>MKKQFATMLAATAVLGVTTAFAANPFSDVTPDSWAYQAVSQLAQAGIVNGYPDGTFKGQNNITRYEMAQMVAKAMANQDRANAEQQAMINRLADEFSNELNNLGVRVSRLEDRVGNVKVTGDARIRYQGSEDKGVYKANSKSLTDGRARVQFNANVNDKTQAVVRVKGNYEFGDSTKGSQATIDRAYVDHKFGSNVSAKAGRFQQTIGGGLMYDDTFDGAQLNVGNDKVQVQGAYGYMIDGAADGNSKSDNPSVSYVGLKGKVGKESSVGGFYSRLSSGNLNHNGVTVNSDKQDVYGFNADFRKNKLWAGGEWLKASNVDNSQAWTAGLGYGNYDIAKKGTWDVKGQYFNQKANAPIVSSTWDQAYDLTNTSNGYKGYMASVDYAVQDNVGLSAGYGFNSKDQSGNDLSDFYRAELNYKFGGHHHHHH[3x]

Most diderm phyla from the Terrabacteria group have recently been shown to lack well-characterised OM attachment systems, but instead have OmpM, which could represent an ancestral tethering system in bacteria. OmpM consists of an N-terminal periplasmic S-layer homology (SLH) domain connected via a linker region to a C-terminal OM β-barrel. Here we use single particle cryo-EM, X-ray crystallography, molecular dynamics simulations, bioinformatic analyses and functional assays to show that OmpM1 from V. parvula (VpOmpM1) is a general porin with similar structural and functional properties to E. coli OmpF, with an additional mobile periplasmic region that can bind V. parvula PG and take on different folds.

The E. coli cell wall does not contain polyaminated PG, the native ligand of VpOmpM1. Therefore, to exclude the possibility that in our structure of VpOmpM1 purified from E. coli the stalk region is misfolded due to the absence of polyaminated PG, we purified a His-tagged OmpM1 construct expressed in V. parvula (native VpOmpM1) and determined its structure by single particle cryo-EM to 3.3 Å resolution. The β-barrel structures are virtually identical (Cα-Cα root-mean-square deviation 0.239 Å), but there are differences in the relative orientation of the stalk. In reconstructions without enforced symmetry, the α-helices forming the coiled-coil are not equivalent in either dataset, as they exit the OM plane in different orientations. A similar interaction was observed in the native VpOmpM1 structure: at two inter-protomer interfaces, R113 interacts with the carbonyl oxygen of G115 and the sidechain of N116 (both part of the β-barrel end of the stalk). Interestingly, the R113-N155 interaction was not observed in the native VpOmpM1 structure, and the R113-G115/N116 interaction was not observed in the VpOmpM1 structure from E. coli. It is possible that the two protein constructs differ slightly in their lowest energy states which are observed in the averaged cryo-EM data. We simulated the native VpOmpM1 model to which an AlphaFold243 prediction of the unmodeled region of the stalk was grafted and fit into the low-resolution cryo-EM density. The simulations revealed substantial movement of the stalk in the periplasmic space. The coiled-coil does not kink throughout the 1 μs simulation, and the movement of the stalk is due to flexibility at the interface between the stalk and the β-barrels.>MVTKIIWVSNNGKPNLKIEFVSEEEKSNFFKEVKKKASELGLNFPLVQGSGNSLLIEASNYPINPCGCYISPGGKLAINFGKVELSHFILPKVGVKTEHAEIFKDHNTIFFHKHKLPGVNSELTFIPTGTPVIVPVTKLEHHHHHH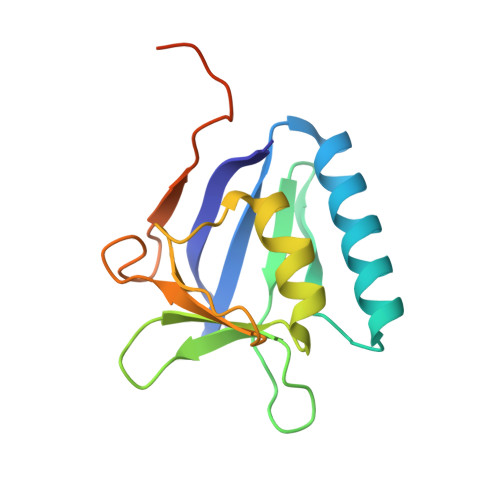[2x]>MEIRKDPFTGEYILVSPHRLKRPWQPEGACPFCPGAPETGRGWDVLILPNRYPVVTENPPEPTAEDLYEVIPARGSSLVVVETPQHDVDDLSDLPL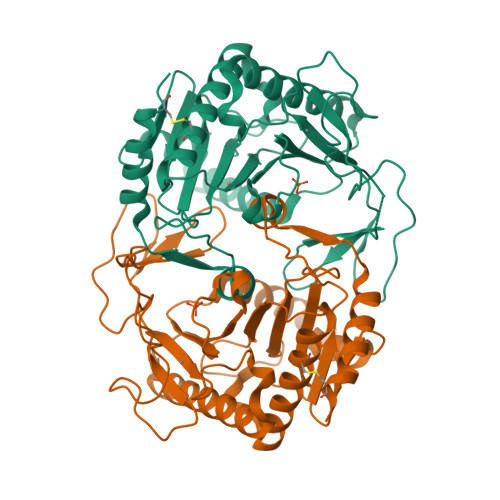GQIKKILTAVAEAQRKAEKEGNAAYFLFFRNKGKEIGVSLTHPHSQIYILPVVPPRVRAELQASYEWYVKHGSCLHCRIVEKEEKRLVFQNRNWKAFVPFYAKWPHEVHIYPKRHRSLLTELTDEEVADLAEALKITLCALKQVAGIPMPYIMVLHQAPLPRPTQYYHLHFEIYGMYRPDGKLKHAAGAELGASLFTLDTTPEETAARIKAALQKCLKHSAD[2x]> GSSKVCRGVIKLSSDCLNKMKLSDFVVLIREKYSYPQDISLLD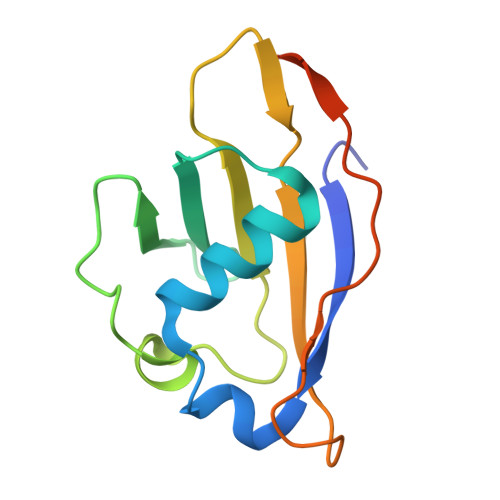ASNQRLLFDYDFEDLNDRTLSEINLGNGSIILFSDEEGDTMIRKAIELFLDVDDELPCNTCSLPDVEVPLIKANNSPSKNEEEE> MLRFPKQVRGGHGTCRVALCSSCRGVALTPQRMQLQHRDRIIGSHGAGLVNHQSMATMEIRSNFTRVQNAAPAADLFRTKVHEGLGTSDKDPYLRTLPNQESRPPESSVLRVAAATAPSLEERQCLHQKWGTLQYWLGDQYPRLPLFLEELLVSDALPVSPAAEAMVQTFAAEVIPAMAKQGGPGAEEKLEALWKQAVQAYGKLTTSHVFDKVAFERELAALRARYQADMSALSPCEDSALALEVLRRKAIAKRNAFLREGLLPMVRNSPYVGYGDGVWRVFFDSVAAHKRDLFSSSNSPVSATLGFAWEGLMMEDAVRTPAMTAPVALYLLLVSISASHNRAPAELKTASAHLDEGIVSTEQRVVPSAFATVSPIVKRRFAADALKGLLGEVKGCGRLAKALRSARLYDWSRDAALCEAMLDDRQLLRADVENMVDRFDSTAEVKSLLQSLMSGTDSAIKAHVSHVFQLPGMASKSHQLVDWDATMSAVDWPHCWREHARELLSDPATLEAVYRLLKNATGAKHATKRLFSDEYAAEVEAALQRRKERAEARKARAEQLVRNLTSYEQVEGTLAVLRKVGVSLRELEGAELATAEQRTVRRPQVDNGVLDLLLEAIRQRHPSWAKSGVLPAVASAAAKSPVWYLECMTRIYIRLSYVPQAAAALMAQRTRRRLGPVGTEPTQFNVPTEMGMVEQYDNLQYKRYDWQGWYQRMVDVHNRNVSIKCRLDDLKRLDAYGNPFVEMQTERRLRILADHRVGMGVLKLDSDKYEDQHDNITYGSTK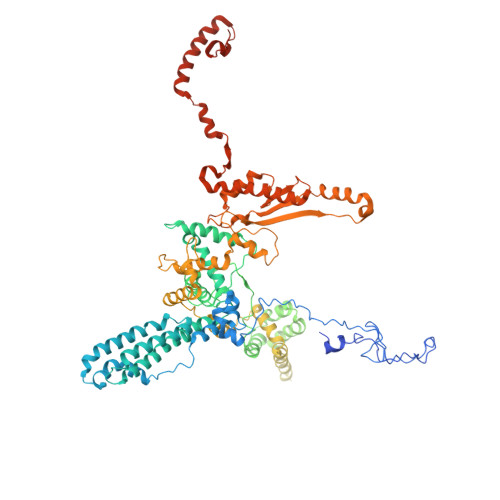LSELLADARKAQLGKEYWPSVEVKVRRPSGQSKAYYSVLDDARIESKSKELYAKYREAKKRSLFVTPMDLWLDVKGMQVRKAAETADAQGYTVDSLQYAMEDDSSDKG> MQRWPKYGGTDVNTRTVHDLLNTINTMSARIKTLERYEHALREIHKVVVILKPSANTHSFEPDALPALIMQFLSDFAGRDINTLTHNINYKYDYNYPPAPVPAMQPPPPPPQPPAPPQPPYYNNYPYYPPYPFSTPPPTQPPESNVAGVGGSQSLNQITLTNEEESELAALFKNMQTNMTWELVQNFVEVLIRIVRVHVVNNVTMINVISSITSVRTLIDYNFTEFIRCVYQKTNIRFAIDQYLCTNIVTFIDFFTRVFYLVMRTNFQFTTFDQLTQYSNELYTRIQTSILQSAAPLSPPTVETVNSDIVISNLQEQLKRERALMQQISEQHRIANERVETLQS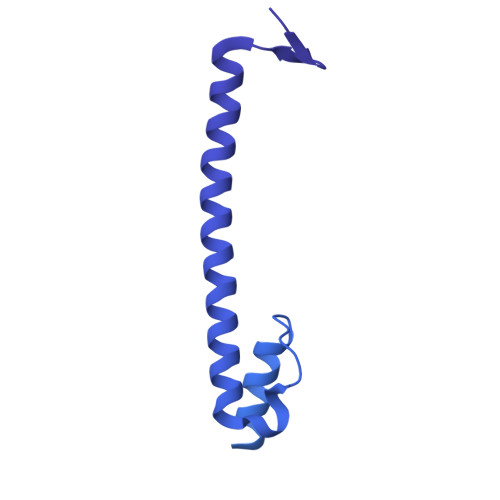QYDELDLKYKEIFEDKSEFAQQKSENVRKIKQLERSNKELNDTVQKLRDENAERLSEIQLQKGDLDEYKNMNRQLNEDIYKLKRRIESTFDKDYVETLNDKIESLEKQLDDKQNLNRELRSSISKIDETTQRYKLDAKDIMELKQSVSIKDQEIAMKNAQYLELSAIYQQTVNELTATKNELSQVATTNQSLFAENEESKVLLEGTLAFIDSFYQIIMQIEKPDYVPISKPQLTAQESIYQTDYIKDWLQKLRSKLSNADVANLQSVSELSDLKSQIISIVPRNIVNRILKENYKVKVENVNAELLESVAVTSAVSALVQQYERSEKQNVKLRQEFEIKLNDLQRLLEQNQTDFESISEFISRDPAFNRNLNDERFQNLRQQYDEMSSKYSALETTKIKEMESIADQAVKSEMSKLNTQLDELNSLFVKYNRKAQDIFEWKTSMLKRYETLARTTAASVQPNVE>MSRSIAQMIDHTLLKPNTTEDQIVKLCEEAKEYSFASVCVNPTWVALAAQLLKDAPDVKVCTVIGFPLGATTPEVKAFETTNAIENGATEVDMVINIGALKDKQYELVGRDIQAVVKAAEGKALTKVIIETSLLTEEEKKAACELAVKAGADFVKTSTGFSGGGATAEDIALMRKVVGPNLG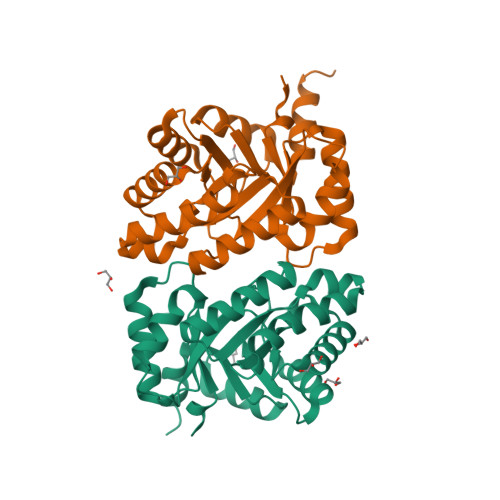VLASGGVRDLSDAKAMIDAGATRIGASAGVAIVNGERSEGSY[6x]> MELPGALQLGELAAAFASVPVFPLFDAAYFIVSVLYLKYEPGAVEMSRKSPFASWLCAMLHCFGSYILADLLLGESPIHYFSNNSSVILATAVWYLIFFCPMNLFYKCVSFLPVKLIFVAMKEVVRVRQIAAGVHHAHHQYHHGWFIMMATGWVKGSGVALMSNFEQLLRGVWRPETNEILHMSFPTKASLYGTVLFTLQQTHWLPVSEANLVFFFTMFMIVCKVFMTAT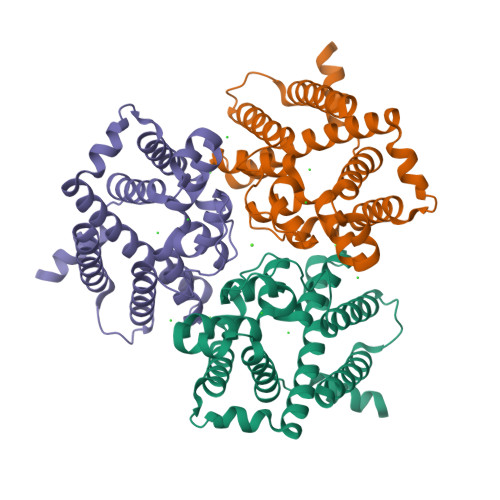HSHASPFAPVEGFISPVFFGSVSSGHTSHHNQHGHSHEASYQPPPPVKSKEELNEGTRKRKAKKAEAAAENLYFQGLEDYKDDDDKHHHHHHHHHH>MDEDGNLQISNSNYNGEEEGEDPENNTLNQPLLKRHRTLSSTPLALVGAKVSHIESLDYEINENDLFKHDWRSRSKAQVFQYIFLKWTLACLVGLFTGLIATLINLAVENIAGYKLLAVGYYIAQDRFWTGLMVFTGANLGLTLVATVLVVYFAPTAAGPGIPEIKAYLNGIDTPNMFGFTTMMVKIVGSIGAVAAGLDLGKEGPLVHIGSCIASLLGQGGPDNHRIKWRWLRYFNNDRDRRDLITCGSASGVCAAFRSPVGGVLFALEEVATWWRSALLWRTFFSTAVVVVVLRAFIEICNSGKCGLFGSGGLIMFDVSHVEVRYHAADIIPVTLIGVFGGILGSLYNHLLHKVLRLYNLINQKGKIHKVLLSLGVSLFTSVCLFGLPFLAECKPCDPSIDEICPTNGRSGNFKQFNCPNGYYNDLSTLLLTTNDDAVRNIFSSNTPNEFGMVSLWIFFGLYCILGLITFGIATPSGLFLPIILMGSAYGRMLGTAMGSYTNIDQGLYAVLGAASLMAGSMRMTVSLCVIFLELTNNLLLLPITMFVLLIAKTVGDSFNLSIYEIILHLKGLPFLEANPEPWMRNLTVGELNDAKPPVVTLNGVEKVANIVDVLRNTTHNAFPVLDGADQNTGTELHGLILRAHLVKVLKKRWFLNEKRRTEEWEVREKFTPVELAEREDNFDDVAITSSEMQLYVDLHPLTNTTPYTVVQSMSVAKALVLFRSVGLRHLLVVPKIQASGMSPVIGILTRQDLRAYNILQAFPHLDKHKSGKAR[2x]

Chloride channels (CLCs) transport anion across membrane to regulate ion homeostasis and acidification of intracellular organelles, and are divided into anion channels and anion/proton antiporters. Arabidopsis thaliana CLCa (AtCLCa) transporter localizes to the tonoplast which imports NO3− and to a less extent Cl− from cytoplasm. The transport mechanism of CLCs has been well established by structural studies which revealed a homodimeric architecture with each protomer bearing a separate ion transport pathway and three consecutive substrate-binding sites referred to as the external site (Sext), central site (Scen) and internal site (Sint). One molecule of ATP and one molecule of PI(4,5)P2 are found binding with each protomer in both structures.

The cryo-EM structure of AtCLCa in complex with Cl− was determined to 3.0 Å (AtCLCa-Cl−), while that in complex with NO3− was determined to 3.2 Å (AtCLCa-NO3−). Moreover, a β-hairpin structure comprised of residues 44–53 is observed in front of the N-terminal loop in each AtCLCa-Cl− protomer, hence, the N-terminal domain (NTD) of AtCLCa is constituted by the β-hairpin, the αA helix and the connecting loop. In the AtCLCa-Cl− structure, αI–J loop covers the ion transport pathway like a lid from the luminal side, whereas in the AtCLCa-NO3− structure, αI–J loop moves away from the ion transport pathway and leaves the ion transport pathway open to the lumen. In the AtCLCa-Cl− structure, three conserved Cl−-binding sites are well-preserved. The Cl− in Sext is coordinated by the main-chain nitrogen of Gly201 on helix αF, as well as Leu479, Phe480, and Leu481 on helix αO. The Cl− in Scen is coordinated by the side chain of Tyr564 on helix αS and main-chain nitrogen of Leu479 on helix αO. The Cl− in Sint is coordinated by the main-chain nitrogen of Gly161 and the side chain of Glu164 on helix αD. The β-hairpin of NTD, firstly identified in our structure, is located below the TMD and occupies the cytoplasmic entrance of the anion transport pathway in each AtCLCa-Cl− protomer. Two small side-chain residues Gly48 and Ala49 constitute the turn of the β-hairpin, and form hydrogen-bonding interactions with the side chains of Glu164 from αD, Lys571 from helix αS and Lys370 from helix αK. The structural information suggests that ATP may function as a molecular glue to stick the NTD and CBS domains together, thus stabilizing the conformation of the β-hairpin to block the anion transport pathway of AtCLCa.> PVNPCCYYPCQHQGICVRFGLDRYQCDCTRTGYSGPNCTIPEIWTWLRTTLRPSPSFIHFLLTHGRWLWDFVNATFIRDTLMRLVLTVRSNLIPSPPTYNIAHDYISWESFSNVSYYTRILPSVPRDCPTPMGTKGKKQLPDAEFLSRRFLLRRKFIPDPQGTNLMFAFFAQHFTHQFFKTSGKMGPGFTKALGHGVDLGHIYGDNLERQYQLRLFKDGKLKYQMLNGEVYPPSVEEAPVLMHYPRGIPPQSQMAVGQEVFGLLPGLMLYATIWLREHNRVCDLLKAEHPTWGDEQLFQTARLILIGETIKIVIEEYVQQLSGYFLQLKFDPELLFGAQFQYRNRIAMEFNQLYHWHPLMPDSFRVGPQDYSYEQFLFNTSMLVDYGVEALVDAFSRQPAGRIGGGRNIDHHILHVAVDVIKESRVLRLQPFNEYRKRFGMKPYTSFQELTGEKEMAAELEELYGDIDALEFYPGLLLEKCHPNSIFGESMIEMGAPFSLKGLLGNPICSPEYWKASTFGGEVGFNLVKTATLKKLVCLNTKTCPYVSFHVPD;> PVNPCCYYPCQHQGICVRFGLDRYQCDCTRTGYSGPNCTIPEIWTWLRTTLRPSPSFIHFLLTHGRWLWDFVNATFIRDTLMRLVLTVQSNLIPSPPTYNIAHDYISWESFSNVSYYTRILPSVPRDCPTPMGTKGKKQLPDAEFLSRRFLLRRKFIPDPQGTNLMFAFFAQHFTHQFFKTSGKMGPGFTKALGHGVDLGHIYGDNLERQYQLRLFKDGKLKY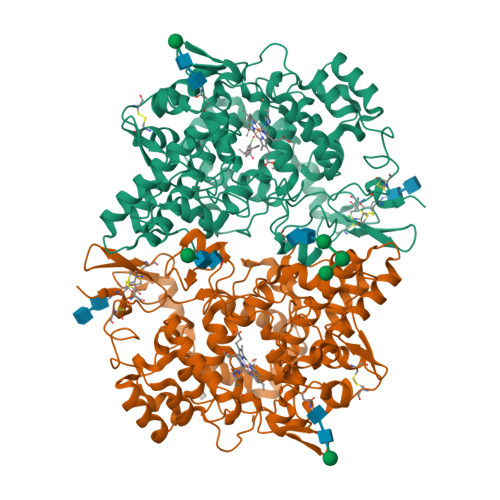QMLNGEVYPPSVEEAPVLMHYPRGIPPQSQMAVGQEVFGLLPGLMLYATIWLREHNRVCDLLKAEHPTWGDEQLFQTARLILIGETIKIVIEEYVQQLSGYFLQLKFDPELLFGAQFQYRNRIAMEFNQLYHWHPLMPDSFRVGPQDYSYEQFLFNTSMLVDYGVEALVDAFSRQPAGRIGGGRNIDHHILHVAVDVIKESRVLRLQPFNEYRKRFGMKPYTSFQELTGEKEMAAELEELYGDIDALEFYPGLLLEKCHPNSIFGESMIEMGAPFSLKGLLGNPICSPEYWKASTFGGEVGFNLVKTATLKKLVCLNTKTCPYVSFHVPD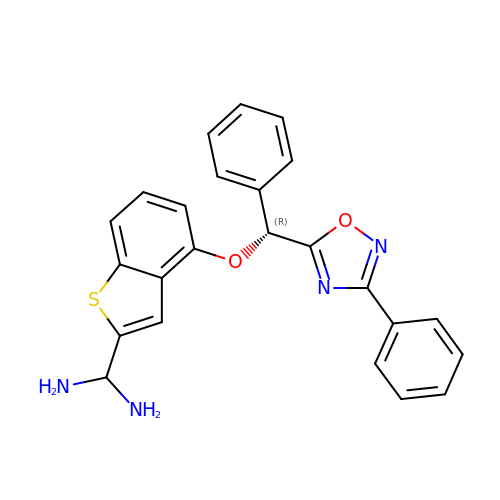1-{4-[(R)-phenyl(3-phenyl-1,2,4-oxadiazol-5-yl)methoxy]-1-benzothiophen-2-yl}methanediamine | C24 H20 N4 O2 S | VBSNODZWDZSFEZ-OAQYLSRUSA-N> MVDCNYSVACNVMVPMRDGVRLAVDLYRPDADGPVPVLLVRNPYDKFDVFAWSTQSTNWLEFVRDGYAVVIQDTRGLFASEGEFVPHVDDEADAEDTLSWILEQAWCDGNVGMFGVSYLGVTQWQAAVSGVGGLKAIAPSMASADLYRAP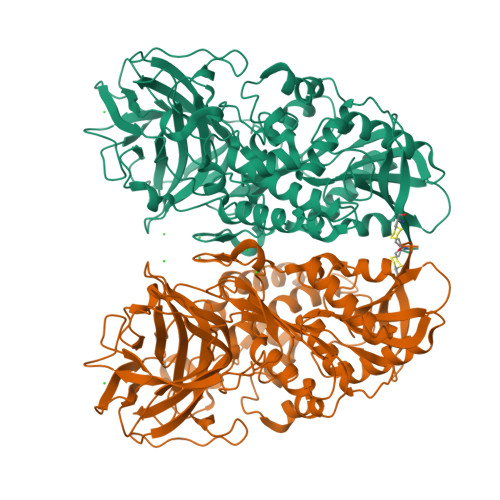WYGPGGALSVEALLGWSALIGTGLITSRSDARPEDAADFVQLAAILNDVAGAASVTPLAEQPLLGRLIPWVIDQVVDHPDNDESWQSISLFERLGGLATPALITAGWYDGFVGESLRTFVAVKDNADARLVVGPWSHSNLTGRNADRKFGIAATYPIQEATTMHKAFFDRHLRGETDALAGVPKVRLFVMGIDEWRDETDWPLPDTAYTPFYLGGSGAANTSTGGGTLSTSISGTESADTYLYDPADPVPSLGGTLLFHNGDNGPADQRPIHDRDDVLCYSTEVLTDPVEVTGTVSARLFVSSSAVDTDFTAKLVDVFPDGRAIALCDGIVRMRYRETLVNPTLIEAGEIYEVAIDMLATSNVFLPGHRIMVQVSSSNFPKYDRNSNTGGVIAREQLEEMCTAVNRIHRGPEHPSHIVLPIIKRKLAAALEHHHHHH5,7-dihydroxy-4-oxo-2-(3,4,5-trihydroxyphenyl)-4H-chromen-3-yl 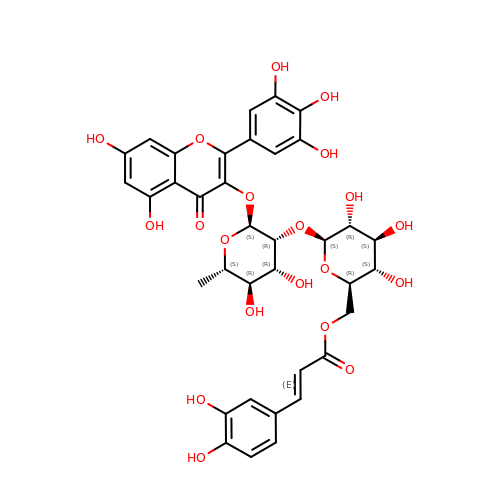6-deoxy-2-O-{6-O-[(2E)-3-(3,4-dihydroxyphenyl)prop-2-enoyl]-beta-D-glucopyranosyl}-alpha-L-mannopyranoside | C36 H36 O20 | YHIHWLPOKDIYGF-ZLGVOOGTSA-N While the spike protein shows extreme diversity and quick adaptation to thwart antibody responses and vaccine effectiveness, the 3C-like main protease (Mpro) has remained relatively conserved. SARS-CoV-2 Mpro also shares the same overall fold and active site with 3C and 3C-like proteases from various coronavirus species and even other viral families. In this work, we report the crystal structures of Mpro from the gamma-CoV SW1 in both apo and inhibitor-bound form, as well as the crystal structure of the delta-CoV HKU15 Mpro in complex with PF-00835231. All four structures were solved with the dimer in the asymmetric unit.

The bisulfite prodrug GC376 converted to the aldehyde form (GC373) and attached covalently to the catalytic Cys142; both active sites were fully occupied by the covalent inhibitor. As previously seen in other Mpro cocrystal structures, the attachment of the aldehyde warhead can result in either (S) or (R)-configuration of the hemithioacetal to orient the hydroxyl group. The electron density was best fit with a 50/50 occupancy of (S)- and (R) configurations at both active sites (in the figures, only the (S) configuration is displayed for clarity). The inhibitor GC376 was bound with the glutamine mimic g-lactam at the P1 position, making direct interactions with Glu163 and inter-ligand stacking with the P3 benzyl ring in one of the protomers. At the active site of the other protomer, the P3 group was flipped such that the benzyl ring interacted with the protease instead of making inter-ligand interactions. The leucine side chain at the P2 position was tucked in the hydrophobic S2 subsite, consistent with the substrate amino acid preference at this position. The P2 group interacts mostly with Glu186, located in the 180s loop. In protomer A, where the P3 moiety bound in the same conformation as in SARS-CoV-2 Mpro, interactions with L162 were less extensive compared to the equivalent M165 while the leucine group of GC376 had considerably higher contacts with Glu186 of SW1 Mpro, compared to Gln189 at the equivalent location in SARS-CoV-2. These interactions were even more pronounced in protomer B where the P3 ring flipped to orient closer to Glu186.

>AGIKKMVAPSSAVEQCVVSVVHGNTQLNGLWLNDYVLCPRHILGKYTGEQWRDALINANNFDFHILYKGMELQVVGRELVGALLKLKVSMVNANTPKYKFAKARIGDNFSIACAYNGHVSGLYTVTLRENGTLKGSFMSGSCGSVGYNVTNEGVEFVYMHHLELPGCVHGGSDLHGIFYGGYVDEEVLQRIPPAPANSRNIVAWLYAAVYNNCDWFVKYGPKQVMSVEDFNEWASGYGFTKFEYHLAFDVFSAATGVSVEQMLAAIKELADGWNYAPVLGSFHLDDEYSPEMIMQQTSGIVLQ[2x]>[2x]QADFEHAISDLEAHNQAKIGVALVSENGNLIQGYRANERFAMCSTFKLPLAALVLSRIDAGEENPERKLHYDSAFLEEYAPAAKRYVATGYMTVTEAIQSALQLSDNAAANLLLKEVGGPPLLTKYFRSLGDKVSRLDRIEPTLNTNTPGDERDTTTPMSMAQTVSKLIFGDTLTYKSKGQLRRLLIGNQTGDKTIRAGLPDSWVTGDKTGS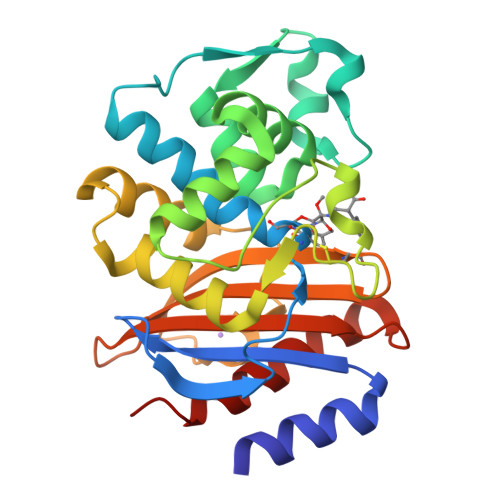CANGGRNDVAFFITTAGKKYVLSVYTNAPELQGEERALLIASVAKLARQYVVH> PEIVDTCSLASPASVCRTKHLHLRCSVDFTRRTLTGTAALTVQSQEDNLRSLVLDTKDLTIEKVVINGQEVKYALGERQSYKGSPMEISLPIALSKNQEIVIEISFETSPKSSALQWLTPEQTSGKEHPYLFSQCQAIHCRAILPCQDTPSVKLTYTAEVSVPKELVALMSAIRDGETPDPEDPSRKIYKFIQKVPIPCYLIALVVGALESRQIGPRTLVWSEKEQVEKSAYEFSETESMLKIAEDLGGPYVWGQYDLLVLPPSFPYGGMENPCLTFVTPTLLAGDKSLSNVIAHEISHSWTGNLVTNKTWDHFWLNEGHTVYLERHICGRLFGEKFRHFNALGGWGELQNSVKTFGETHPFTKLVVDLTDIDPDVAYSSVPYEKGFALLFYLEQLLGGPEIFLGFLKAYVEKFSYKSITTDDWKDFLYSYFKDKVDVLNQVDWNAWLYSPGLPPIKPNYDMTLTNACIALSQRWITAKEDDLNSFNATDLKDLSSHQLNEFLA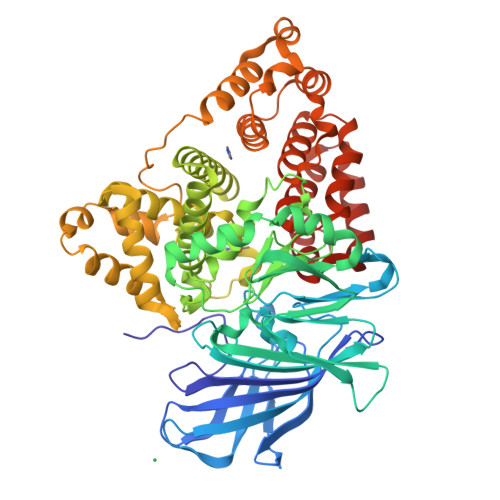QTLQRAPLPLGHIKRMQEVYNFNAINNSEIRFRWLRLCIQSKWEDAIPLALKMATEQGAMKFTRPLFKDLAAFDKSHDQAVRTYQEHKASMHPVTAMLVGKDLKVD Ovalbumin-related protein X belongs to the serpin family (SERine Protease INhibitor, I4) and more precisely to the subgroup clade B serpins, also known as ov-serpins. Similar to ovalbumin, OVAX lacks inhibitory activity against serine proteases and little is known regarding its physiological functions. However, OVAX possesses antibacterial activity against Listeria monocytogenes and S. Enteritidis, and this activity is blocked in the presence of heparin glycosaminoglycan. Although OVAX is mainly expressed in the magnum (responsible for egg white formation), it was identified in the eggshell and its relative abundance (emPAI) was elevated in uterine fluid during the terminal phase of eggshell formation (45th based on EmPAI value).

A cationic domain present in OVAX, but not in ovalbumin or in OVAY structures, is likely to be responsible for this antibacterial activity, as it could explain the interaction of OVAX with the negatively charged bacterial cell wall. X-ray structural analysis of OVAX complexed to Fondaparinux (a synthetic pentasaccharide derived from heparin) confirms the ability of OVAX to bind glycosaminoglycans in a region that is close to the cationic domain that was initially predicted to bind heparin. This pentasaccharide interacts via a network of hydrogen bonds involving Gly57, Asn58, Glu64 of OVAX and a salt bridge formed between the Arg56 side chain with a sulfate group of the pentasaccharide. The Fondaparinux binding site of OVAX contains both negatively and positively charged areas at the top of the molecule as depicted. The role of OVAX in eggshell formation has not been explored yet but it is noteworthy that its paralog ovalbumin modifies calcium carbonate crystallization and potentially plays a role in ACC stabilization and eggshell calcification. This mechanism of action of ovalbumin possibly involves acidic amino acids that would bind Ca2+ cations. The analysis of OVAX structure also reveals the presence of several negatively charged regions. This observation, together with the capacity of OVAX to bind heparin and possibly eggshell glycosaminoglycans, should stimulate studies to further explore its role in eggshell mineralization. For certain proteins (OC-17, VMO1, OCX-32, OVAX, Ex-FABP), 3D structure analysis reveals a clear bipolar distribution of negative and positive charges on their molecular surface. In addition, five of these eggshell antimicrobial proteins bind glycosaminoglycan moieties (VMO1, AvBD11, OVAX, MSMB3 and pleiotrophin), which opens new research avenues to explore their interactions with avian eggshell glycosaminoglycans and proteoglycans.

> MFFYNTDFRMGSISAANAEFCFDVFNELKVQHTNENILYSPLSIIVALAMVYMGARGNTEYQMEKALHFDSIAGLGGSTQTKVQKPKCGKSVNIHLLFKELLSDITASKANYSLRIANRLYAEKSRPILPIYLKCVKKLYRAGLETVNFKTASDQARQLINSWVEKQTEGQIKDLLVSSSTDLDTTLVLVNAIYFKGMWKTAFNAEDTREMPFHVTKEESKPVQMMCMNNSFNVATLPAEKMKILELPFASGDLSMLVLLPDEVSGLERIEKTINFEKLTEWTNPNTMEKRRVKVYLPQMKIEEKYNLTSVLMALGMTDLFIPSANLTGISSAESLKISQAVHGAFMELSEDGIEMAGSTGVIEDIKHSPELEQFRADHPFLFLIKHNPTNTIVYFGRYWSP2,7-dimethyl-6-[(prop-1-yn-1-ylamino)methyl]quinazolin-4(3H)-one 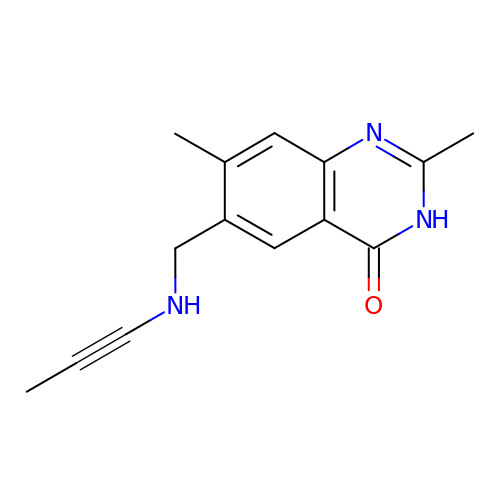| C14 H15 N3 O | VHJQNTIPWBTKDM-UHFFFAOYSA-N>AADIVQMVEDLTGKLTALAWALFLLSWSIGWTLRGSPIPSSRIKRVGNSLIEDSMWAALWLALGT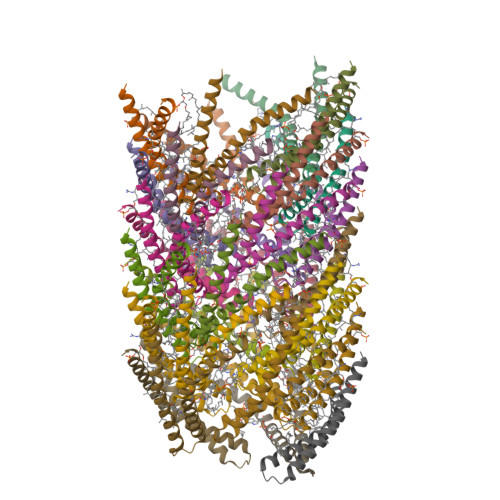TVFAVIVRLAGIVNEVLLG[30x]2-(4-CARBAMIMIDOYL-2-HYDROXY-BENZYLAMINO)-PROPIONIC 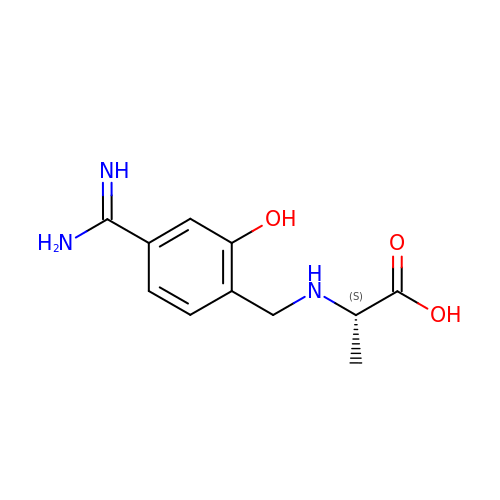ACID | C11 H15 N3 O3 | DQRWCBYLVLYBIF-LURJTMIESA-N> MTDLIQRPRRLRKSPALRAMFEETTLSLNDLVLPIFVEEEIDDYKAVEAMPGVMRIPEKHLAREIERIANAGIRSVMTFGISHHTDETGSDAWREDGLVARMSRICKQTVPEMIVMSDTCFCEYTSHGHCGVLCEHGVDNDATLENLGKQAVVAAAAGADFIAPSAAMDGQVQAIRQALDAAGFKDTAIMSYSTKFASSFYGPFREA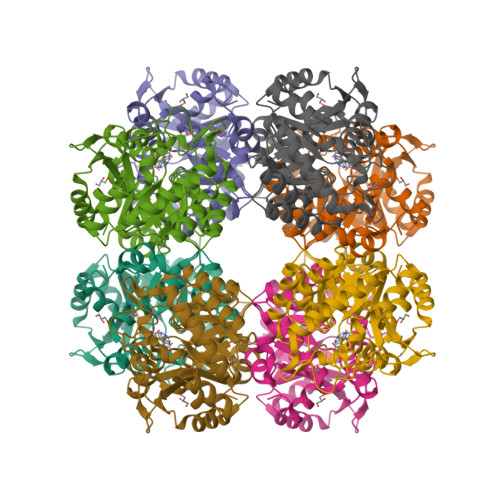AGSALKGDRKSYQMNPMNRREAIRESLLDEAQGADCLMVKPAGAYLDIVRELRERTELPIGAYQVSGEYAMIKFAALAGAIDEEKVVLESLGSIKRAGADLIFSYFALDLAEKKILR> AAASNKDAALLEAARANNMQEVSRLLSEGADVNAKHRLGWTALMVAAINRNNSVVQVLLAAGADPNLGDDFSSVYKTAKEQGIHSLEDGGQDGASRHITNQWTSALEFRRWLGLPAGVLITREDDFNNRLNNRASFKGCTALHYAVLADDYRTVKELLDGGANPLQRNEMGHTPLDYAREGEVMKLLRTSEAKYQEKQRKREAEERRRFPLEQRLKEHIIGQ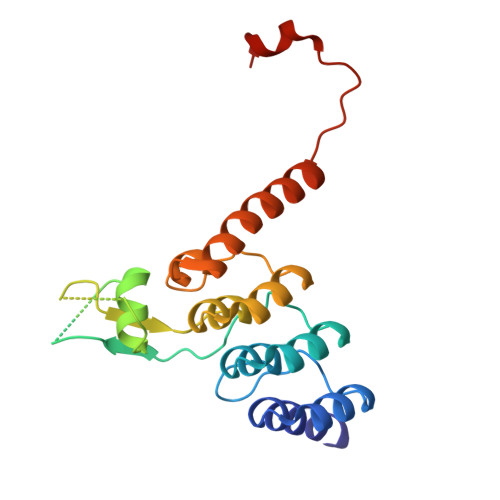E>[2x]MPRYLGLMSGTSLDGMDIVLIEQGDRTTLLASHY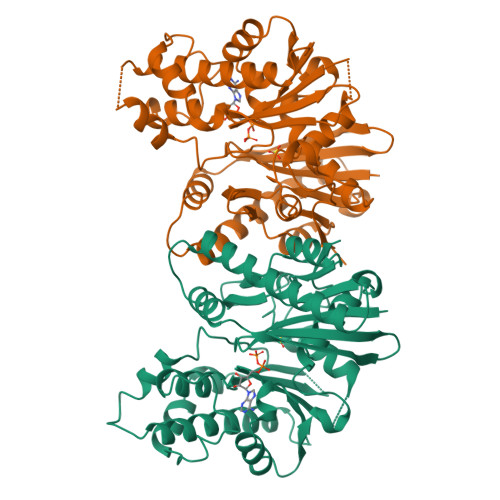LPMPAGLREDILALCVPGPDEIARAAEVEQRWVALAAQGVRELLLQQQMSPDEVRAIGSHGQTIRHEPARHFTVQIGNPALLAELTGIDVVADFRRRDVAAGGQGAPLVPAFHQALFGDDDTSRAVLNIGGFSNVSLLSPGKPVRGFDCGPGNVLMDAWIHHQRGEHFDRDGAWAASGQVNHALLASLLADEFFAARGPKSTGRERFNLPWLQEHLARHPALPAADIQATLLELSARSISESLLDAQPDCEEVLVCGGGAFNTALMKRLAMLMPEARVASTDEYGIPPAWMEGMAFAWLAHRFLERLPGNCPDVTGALGPRTLGALYPAGSHHHHHH>SGFVCNTCPEKWINFQRKCYYFGKGTKQWVHARYACDDMEGQLVSIHSPEEQDFLTKHASHTGSWIGLRNLDLKGEFIWVDGSH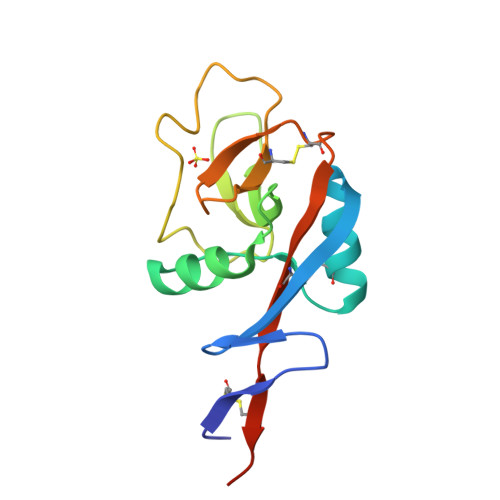VDYSNWAPGEPTSRSQGEDCVMMRGSGRWNDAFCDRKLGAWVCDRLATCTPPASEGSAE[4x]>[2x]MGKAVIAIHGGAGAISRAQMSLQQELRYIEALSAIVETGQKMLEAGESALDVVTEAVRLLEECPLFNAGIGAVFTRDETHELDACVMDGNTLKAGAVAGVSHLRNPVLAARLVMEQSPHVMMIGEGAENFAFARGMERVSPEIFSTSLRYEQLLAARKEGATVLDHSGAPLDEKQKMG;>TVGAVALDLDGNLAAATSTGGMTNKLPHTVGPQPLVGAGCYANNASVAVSCTGTGEVFIRALAAYDIAALMDYGGLSLAEACERVVMEKLPALGGSGGLIAIDHEGNVALPFNTEGMYRAWGYAGDTPTTGIYREKGDTVATQ[2x]

l-Asparaginases hydrolyze l-asparagine to l-aspartic acid and ammonia. The prototypic class 2 enzyme is EcAIII from E. coli. EcAIII belongs to the Ntn-hydrolases, which are expressed as immature polypeptides that dimerize and then autocatalytically cleave themselves into α (∼20 kDa) and β (∼15 kDa) subunits to form the mature (αβ)2 heterotetramer (a dimer of two αβ heterodimers). The same Thr179 acts as the nucleophile in the autoproteolytic maturation and in l-asparagine hydrolysis.

Variant RDM1-3, in addition to the R207T substitution, also carries a G206H mutation. The side chain of His206 is exposed outside the active site and occupies the space between Glu81, Glu125 and Gly126. Thr207 is hydrogen-bonded to the carbonyl O atom of Pro204, and this interaction stabilizes the entire 200–208 loop. Two other substitutions, D210P and S211Q, located closer to the nucleophilic Thr179, do not affect the conformation of the neighboring residues. The relatively long side chain of Gln211 fits well into a cleft surrounded by Thr179, Thr230 and Pro210, and forms a hydrogen bond to the Oγ1 atom of Thr195 and the carbonyl O atom of Cys229. Waters w3 and w4 are absent in variants with bulky side chains at position 211, such as Gln (RDM1-3) or Trp (RDM1-18). Asp210 and Ser211 could be substituted individually (variant RDM1-37, D210S mutation only) or simultaneously (variants RDM1-3, RDM1-8, RDM1-12, RDM1-18, RDM1-24, RDM1-29 and RDM1-38) without any loss of autocatalytic activity.>MGSSHHHHHHSSGLVPRGSHMSSSGDARPSQKGILLPAARANDTDEAAGRRSIAWPVARTCPFSPPEQYAALRAEEPIARAELWDGAPVWLISRQDHVRALLADPRVSIHPAKLPRLSPSDGEAEASRSLLTLDPPDHGALRGHFIPEFGLRRVRELRPSVEQIVTGLLDDLTARGDEADLLADFALPMATQVICRLLDIPYEDRDYFQERTEQATRPAAGEEALEALLELRDYLDRLISGKTGRESGDGMLGSMVAQARGGGLSHADVLDNAVLLLAAGHETTASMVTMSVLVLLQHPTAWRELTVNPGLLPGAVDELLRYLSIADGLRRSATADIEIDGHTIRAGDGLVFLLAAANRDEAVFSEP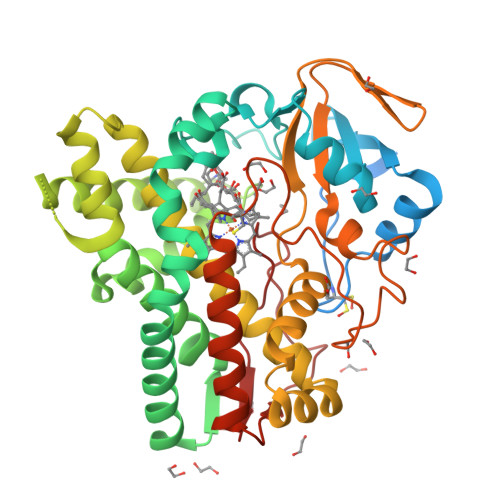EAFDIHRSARRHVAFGYGPHQCLGQNLARMELEVALGAVLERLPALRPTTDVAGLRLKSDSAVFGVYELPVAW[2x]> VVEAVENAVARVADTISSGPSNSQAVPALTAV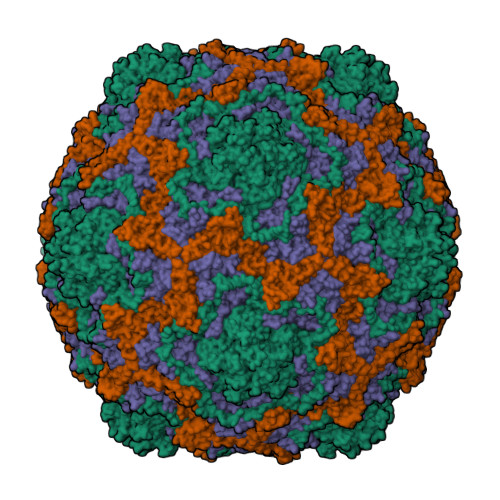ETGHTSQVTPSDTIQTRHVRNYHSRSESSIENFLCRSACVYMGEYHTTNTDTSKLFASWTINARRMVQMRRKLELFTYVRFDMEVTFVITSKQDQGTQLGQDMPPLTHQIMYIPPGGPIPKSVTDYTWQTSTNPSIFWTEGNAPPRMSIPFISIGNAYSNFYDGWSHFSQNGVYGYNTLNHMGQIYVRHVNGSSPLPMTSTVRMYFKPKHVKVWVPRPPRLCQYKNASTVNFTPTNITEKRQSINYIPETVKP;> DRVRSITLGNSTITTQESANVVVAYGRWPEYLKDNEATAEDQPTQPDVATCRFYTLESVTWERDSPGWWWKFPDALKDMGLFGQNMYYHYLGRAGYTIHVQCNASKFHQGCLMVVCVPEAEMGCSQVDGTVNEHSLSEGETAKKFASTSTNGTNTVQSIVTNAGMGVGVGNLTIFPHQWINLRTNNCATIVMPYINNVPMDNMFRHHNFTLMIIPFVPLDYSSDSSTYVPITVTVAPMCAEYNGLRLATSL;> GLPVMNTPGSNQFLTSDDFQSPSAMPQFDVTPELNIPGEVQNLMEIAEVDSVVPVNNVEGKLDTMEIYRIPVQSGNHQSSQVFGFQVQPGLDNVFKHTLLGEILNYYAHWSGSIKLTFVFCGSAMATGKFLLAYAPPGANAPKSRKDAMLGTHIIWDVGLQSSCVLCIPWISQTHYRLVQQDEYTSAGNVTCWYQTGIVVPAGTPTSCSIMCFVSACNDFSVRLLKDTPFIEQSALLQ;> MGAQVSTQKTGAHETGLNASGRSIIHYTNINYYKDAASNSANRQDFSQDPGKFTEPVKDIMVKSLPALN N-[4,5,7-TRICARBOXYHEPTANOYL]-L-GAMMA-GLUTAMYL-N-{2-[4-({5-[(FORMYLAMINO)METHYL]-3-FURYL}METHOXY)PHENYL]ETHYL}-D-GLUTAMINE 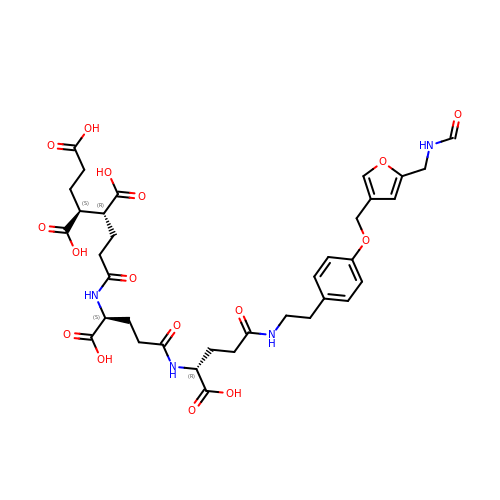| C35 H44 N4 O16 | RGBIJPWAWLXPOC-XRVZLLLRSA-N> MEDISTEKTVESLEAIRHRIAQIV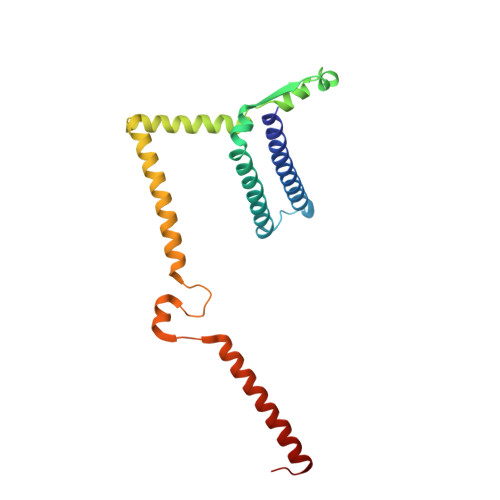QSLTHFLAILHQSESLSPWPTIHKNFNILLSQIHSLSNNLAAHSHTLQTTSIYPSLEFPVKEQEPLLTTLLRTKALPEVEEWEANTLQEYEASISSQPKKKEANDAYQKDQLWDQARIIFMEERENYSWFDFVTRRQESEGEFVSQRQLEIDRATEEQNANQMLTDILSFMKSGKR Eravacycline | C27 H31 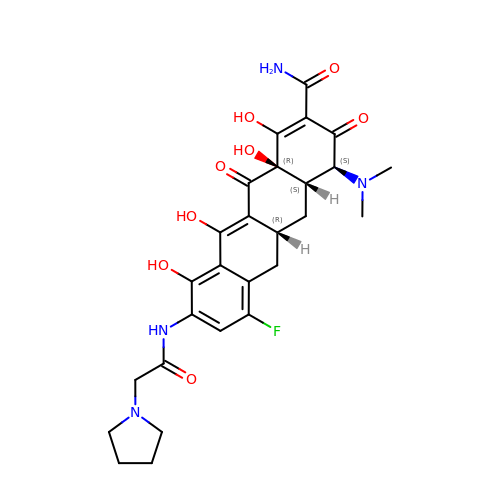F N4 O8 | AKLMFDDQCHURPW-ISIOAQNYSA-N> HKIL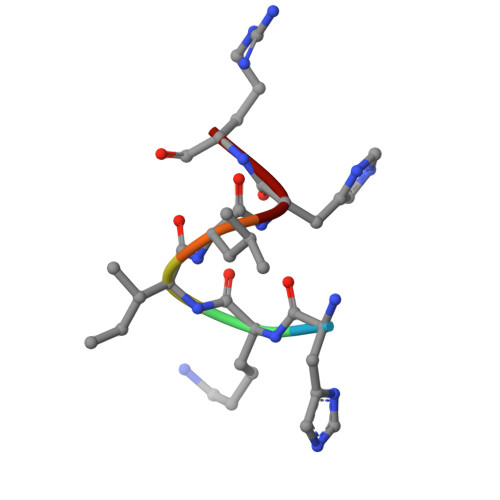HR PNGM-1 is derived from a metagenomic library from deep-sea sediments that predate the antibiotic era. PNGM-1 has both MBL and tRNase Z activities and is considered to be the evolutionary origin of B3 MBLs. The wild-type of PNGM-1 has two MBSs in its substrate-binding pocket, and each is occupied by a zinc ion. The zinc ion in the first MBS (Zn1) is coordinated by the residues His91, His93, His188, and Asp210; the zinc ion in the second MBS (Zn2), by Asp95, His96, His279, and Asp210.

His91 and His93 coordinate the zinc ion at Zn1, whereas His96 and His279 coordinate that at Zn2. In the crystal structures of the H96A and H279A variants, the electron density of the zinc ion at Zn2 is markedly lower compared to that in the wild-type structure, indicating that either a water molecule with full occupancy or a zinc ion with half occupancy is present in this site. The residues His93, Aps95, His279, and Asp210 occupy equatorial positions along the enzyme’s surface. In the structures of all PNGM-1 variants, except in that of H96A, the electron density corresponding to the catalytic water remains despite the complete or partial loss of a zinc ion. Each MBS of PNGM-1 is formed by four metal-coordinating residues, and the substitution of only one of these residues dramatically reduces the metal binding affinity of the enzyme.

>AGGKVTSSTGIAPKRYVYYPGSEELGPDEIRVIACGTGMPTARRAQAAAAWVVELGNGDKFIVDIGSGSMANIQSLMIPANYLTKIFLTHLHTDHWGDLVSMWAGGWTAGRTDPLEVWGPSGSREDMGTKYAVEHMLKAYNWDYMTRAVTINPRPGDINVHEFDYRALNEVVYQENGVTFRSWPCIHAGDGPVSFALEWNGYKVVFGGDTAPNIWYPEYAKGADLAIHECWMTSDQMMTKYNQPAQLALRINLDFHTSAQSFGQIMNMVQPRHAVAYAFFNDDDTRYDIYTGVRENYAGPLSMATDMMVWNITRDAVTERMAVSPDHAWDVAGPSEDLAPDRNRASEYTQYILDGRLNVDEANAHWKQEFMG[4x]>[4x]MTHHYPTDDIKIKEVKELLPPIAHLYELPISKEASGLVHRTRQEISDLVHGRDKRLLVIIGPCSIHDPKAALEYAERLLKLRKQYENELLIVMRVYFAKPRTTVGWKGLINDPHLDGTFDINFGLRQARSLLLSLNNMGMPASTEFLDMITP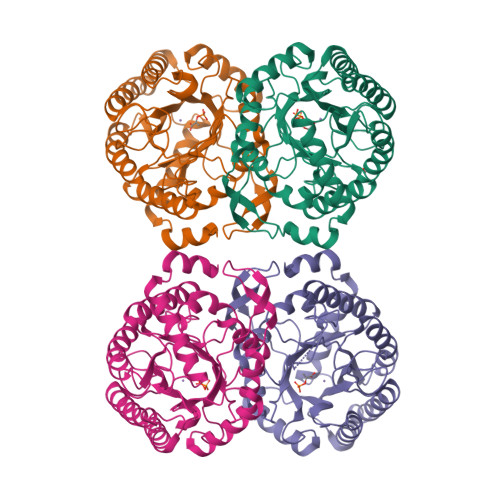QYYADLISWGAIGARTTESQVHRELASGLSCPVGFKNGTDGNLKIAIDAIGAASHSHHFLSVTKAGHSAIVHTGGNPDCHVILRGGKEPNYDAEHVSEAAEQLRAAGVTDKLMIDCSHANSRKDYTRQMEVAQDIAAQLEQDGGNIMGVMVESHLVEGRQDKPEVYGKSITDACIGWGATEELLALLAGANKKRMARAS> SRSESSIENFLCRAACVYYATYTNNSEKGYAEWVINTRQVAQLRRKLELFTYLRFDLELTFVITSAQQPSTATSVDAPVQTHQIMYVPPGGPVPTKVTDYAWQTSTNPSVFWTEGNAPPRMSIPFISIGNAYSCFYDGWTQFSRNGVYGINTLNNMGTLYMRHVNEAGQGPIKSTVRIYFKPKHVKAWVPRPPRLCQYEKQKNVNFTPTGVTTTRVGITT;> RVRSITLGNSTITTQECANVVVGYGVWPEYLKDNEATAEDQPTQPDVATCRFYTLESVQWMKNSAGWWWKLPDALSQMGLFGQNMQYHYLGRTGYTIHVQCNASKFHQGCLLVVCVPEAEMGCSNLNNTPEFAELSGGDTARMFTDTQIGETNSKKVQTAVWNAGMGVGVGNLTIYPHQWINLRTNNSATIVMPYINSVPMDNMFRHNNLTLMIIPFVPLNYSEGSSPYVPITVTIAPMCAEYNGLRLA;> GLPVMTTPGSTQFLTSDDFQSPSAMPQFDVTPEMQIPGRVNNLMEIAEVDSVVPVNNTEANVNSLKAYQIPVQSNSDNGKQVFGFPLQPGANGVLNRTLLGEILNYYTHWSGSIKLTFMFCGSAMATGKFLLAYSPPGAGVPKNRKDAMLGTHVIWDVGLQSSCVLCVPWISQTHYRYVVEDEYTAAGYITCWYQTNIVVPADVQSSCDILCFVSACNDFSVRMLKDTP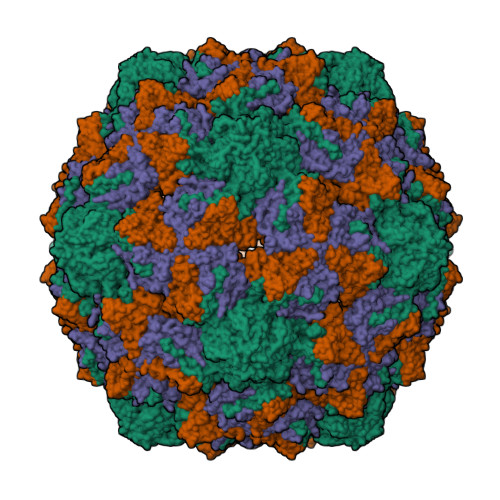FIR>[4x]MPVPNGATFPPCARKMERADGPATVLAIGTANPPNVFDQSTYPDFYFNITNSNHMTDLKTKFQRMCDKSGIT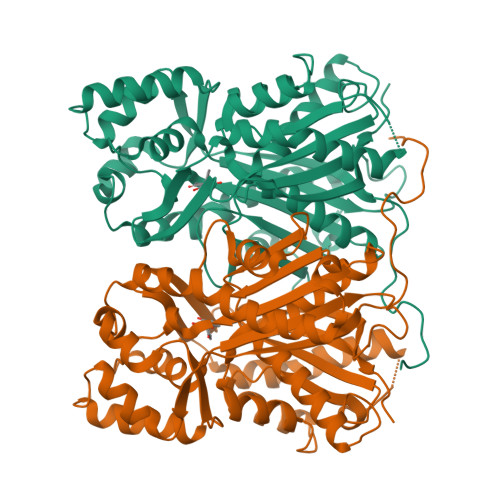KRYMYLNEEILKANPNMCAYWEKSLDVRQDMVVVEVPKLGKEAATKAIKEWGQPKSKITHVVFCTTSGVDMPGADWALTKLLGLRPSVKRLMMYQQGCFAGGTVMRVAKDLAENNKGARVLVVCSELTAVTFRGPSETHLDSLVGQALFGDGASAIIVGADPIPEVERPWFEIHYVASNILPDSDGAIDGHLREVGLTFHLMKDVPGIISKNIGTVLKDAFEKVFGNEEGEVPSYNDVFWIAHPGGPAILDQVEQKLQLKTEKMAASRQVLSDYGNMSSACVLFIMDHLRKKSVEQKLATSGEGYEWGLLLGFGPGLTCETVVLRSVPLATE[(5R)-5-(2,3-dibromo-5-ethoxy-4-hydroxybenzyl)-4-oxo-2-thioxo-1,3-thiazolidin-3-yl]acetic acid | C14 H13 Br2 N O5 S2 | 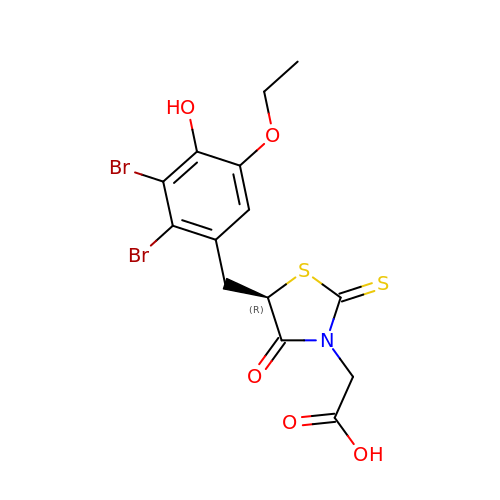ABQHPGHMYXJJIV-MRVPVSSYSA-N>DNPIDSCWRGDSNWDQNRMKLADCAVGFGSSTMGGKGGDFYTVTSTDDNPVNPTPGTLRYGATREKALWIIFSQNMNIKLKMPLYVAGHKTIDGRGADVHLGNGGPCLFMRKVSHVILHSLHIHGCNTSVLGDVLVSESIGVEPVHAQDGDAITMRNVTNAWIDHNSLSDCSDGLIDVTLGSTGITISNNHFFNHHKVMLLGHDDTYDDDKSMKVTVAFNQFGPNAGQRMPRARYGLVHVANNNYDPWNIYAIGGSSNPTILSEGNSFTAPSESYKKEVTKRIGCESPSACANWVWRSTRDAFINGAYFVSSGKTEETN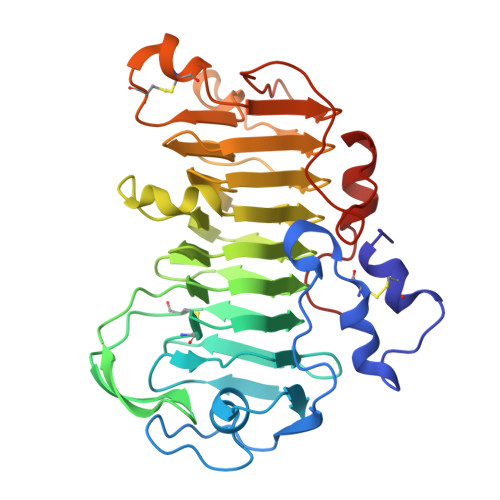IYNSNEAFKVENGNAAPQLTKNAGVVT[2x]>GSHMTVPTWQVRDLRRILRVSELSQHLRQARTDFRSTLSQLVYFNRSVVNPNEYDDEYLLSDQRLTYVYVDEVTAQLCGLNRLLPSNSPAFGTVATAMPPWLLDPQEMNAILQQSCGQGGFVNYHHGPSTNGFFLAILMSQLFIRIRTDVIRGQGYGWYARQGNYVEEGEDNEGIENEEEE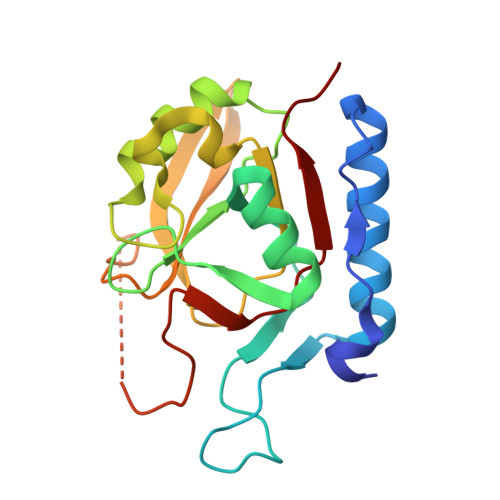EETREFQLSDLIHYPIVALGSCHLTR[2x]> GELVRTDSPNFLCSVLPTHWRCNKT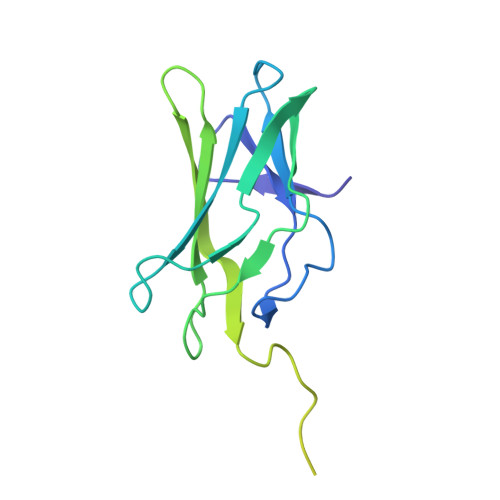LPIAFKVVAKGDVPDGTLVTVMAGNDENYSAELRNATAAMKNQVARFNDLRFVGRSGRGKSFTLTITVFTNPPQVATYHRAIKITVDGPREPRRHRQKLDDQTKPGSLSFSERLSELEQLRRTAMRVSPHHPAPTPNPRASLNHSTAFNPQPQSQMQDARQIQPSPPWSYDQSYQYLGS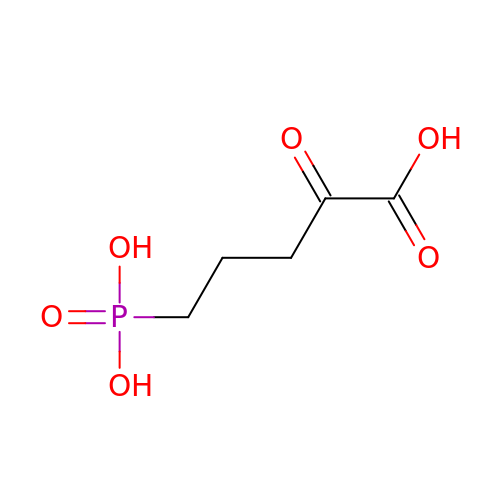2-OXO-5-PHOSPHONOPENTANOIC ACID | C5 H9 O6 P | UFXCSKVWNXIICO-UHFFFAOYSA-N> MKTDFNQKIEQLKEFIEECRRVWLVLKKPTKDEYLAVAKVTALGISLLGIIGYIIHVPATYI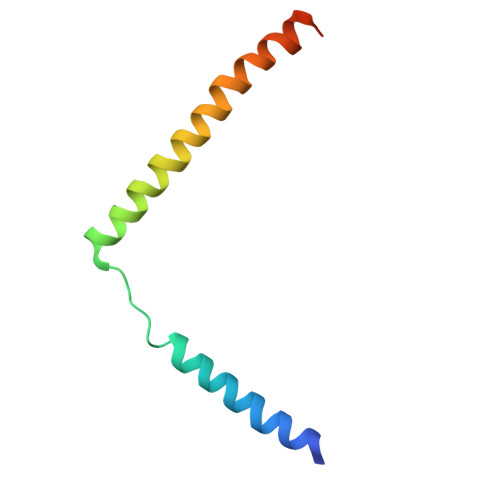KGILKPPTTPRV>MSNKCDVVVVGGGISGMAAAKLLHDSGLNVVVLEARDRVGGRTYTLRNQKVKYVDLGGSYVGPTQNRILRLAKELGLETYKVNEVERLIHHVKGKSYPFRGPFPPVWNPITYLDHNNFWRTMDDMGREIPSDAPWKAPLAEEWDNMTMKELLDKLCWTESAKQLATLFVNLCVTAETHEVSALWFLWYVKQCGGTTRIFSTTNGGQERKFVGGSGQVSERIMDLLGDRVKLERPVIYIDQTRENVLVETLNHEMYEAKYVISAIPPTLGMKIHFNPPLPMMRNQMITRVPLGSVIKCIVYYKEPFWRKKDYCGTMIIDGEEAPVAYTLDDTKPEGNYAAIMGFILAHKARKLARLTKEERLKKLCELYAKVLGSLEALEPVHYEEKNWCEEQYSGGCYTTYFPPGILT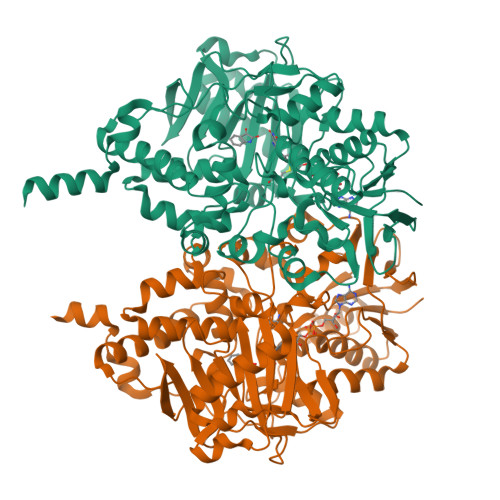QYGRVLRQPVDRIYFAGTETATHWSGYMEGAVEAGERAAREILHAMGKIPEDEIWQSEPESVDVPAQPITTTFLERHLPSVPGLLRLIGLTTIFSATALGFLAHKRGLLVRV[2x]CAD is a 1.5 MDa hexameric protein with four enzymatic domains responsible for initiating de novo biosynthesis of pyrimidines nucleotides: glutaminase, carbamoyl phosphate synthetase, aspartate transcarbamoylase (ATC), and dihydroorotase. Moreover, in fungi, GLN, CPS, and ATC are fused into a CAD-like protein with an inactive DHO-like domain, and the DHO activity is encoded as an independent enzyme. The crystal structures of the ATC domains of human CAD and the CAD-like protein from the fungus Chaetomium thermophilum showed a dome-shaped homotrimer with three active sites between the subunits that are very similar to bacterial and plant ATCs. Here, we report the insertion by site-directed mutagenesis of two cysteine (Cys) residues in the ATC domain that favor the formation of disulfide bridges between subunits in the trimer.

So, for this study, we engineered a construct encoding only the ctATC domain (ctATC-WT; aa 1939–2253) fused to a removable N-terminal His6-maltose binding protein (MBP) tag and then introduced the mutations N2045C and R2238C (ctATC2Cys). Using these criteria, we selected residue N2045, in helix α3, and residue R2238, in helix α12. Indeed, similar ctATC2Cys crystals grown with CP showed extra electron density at the active site assigned to the bound substrate and residues S2029 and K2032 from the CP-loop, which was well-defined in this structure. The binding of CP to ctATC2Cys was as already described for ctATC-WT, including a small hinge closure of the protein subunit. The only important difference in the structures of ctATC2Cys that are free or bound to CP was the presence of the mutated Cys residues and the extra electron density between their side chains that demonstrates the formation of three disulfide bridges between subunits in the trimer. Thus, we conclude that the Cys and formation of the disulfide bridges do not alter the protein folding or oligomerization and do not interfere with the binding of CP. The high-resolution crystal structures of ctATC2Cys also indicate that the disulfide bridge does not alter protein folding and neither impedes the binding of CP nor the induced conformational changes. However, we could not grow crystals of ctATC2Cys in complex with PALA (N-phosphonoacetyl-L-aspartate), a transition state analog that induces a large conformational change of the Asp-domain that is required for the reaction. On the other hand, the activity assays with ctATC2Cys showed that the mutations to Cys increased the activity of the enzyme, making it two-fold faster than the ctATC-WT (v = 8.87 ± 1.06 mmoles·h−1·mg−1). Overall, these assays indicated that disulfide bond formation, rather than hampering protein activity, increases the specific activity, most likely by preventing dissociation of the active trimer at the high dilutions used for the assay.

> SPLQEMLAAPSSFKKSHVLSVTQFTRADLHLLFQIAQEMRLGVQREGVLDILRGKVLCTLFYEPSTRTSASFDAAMQRLGGRTIPIQTSTSSVQKGETLQDTLRTLACYSDAIVLRHPDEKCVDVAKKYCPVPVINGGNGSKEHPTQAFLDLFTIREELGTMQGLTITFVGDLLYGRPVHSLVYLLRHYQVKVQLVSPKALRLPPAVRQQLVDAGQLLCESEALTPEILGRTDVLYCTRVQKERFPSLAEFEAVKDSYRIDYSTLKYAKPTTVVMHPLPRNEEVAEEVDFDQRAAYFRQMCYGLYCRMALLALVMS4-(4-methylpiperazine-1-sulfonyl)benzamide | C12 H17 N3 O3 S | 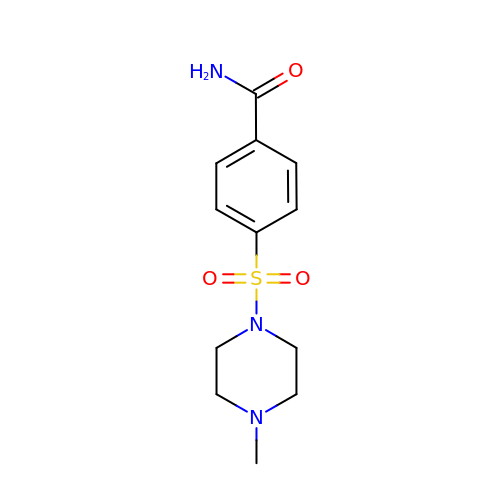DGYBGNBRDCUNEP-UHFFFAOYSA-N> GHMERLLDELTLEGVARYMQSERCRRVICLVGAGISTSAGIPDFRSPSTGLYDNLEKYHLPYPEAIFEISYFKKHPEPFFALAKELYPGQFKPTICHYFMRLLKDKGLLLRCYTQNIDTLERIAGLEQEDLVEAHGTFYTSHCVSASCRHEYPLSWMKEKIFSEVTPKC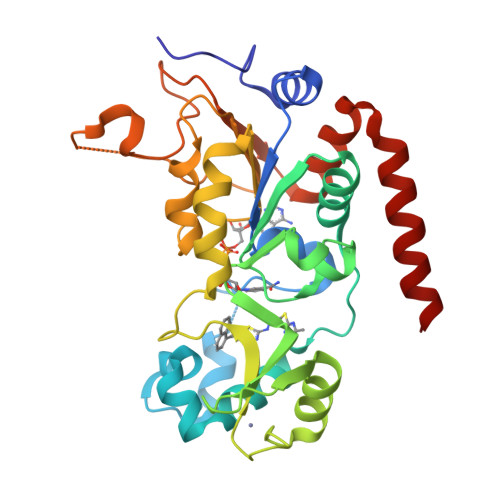EDCQSLVKPDIVFFGESLPARFFSCMQSDFLKVDLLLVMGTSLQVQPFASLISKAPLSTPRLLINKEKAGQSDPFLGMIMGLGGGMDFDSKKAYRDVAWLGECDQGCLALAELLGWKKELEDLVRREHASIDAQS>[2x]SLVELGKMILQETGKNPVKSYGAYGCNCGVLGRGKPKDA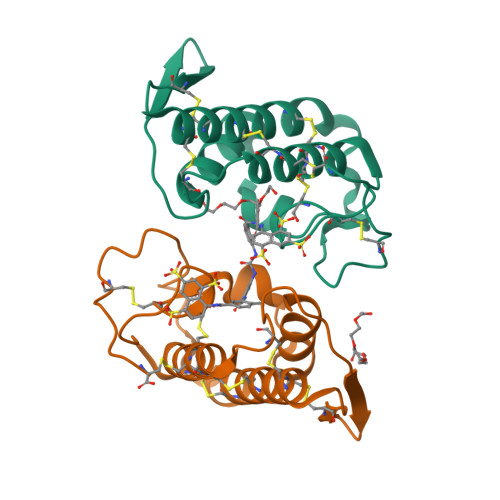TDRCCYVHKCCYKKLTNCNPKKDRYSYDWKNKTIVCGEENPCLKQLCECDKAVAICLRENKGTYNKKRDVYLKPFCDKGRDC> TDLSQRPRRLRKSPALRAMFEETTLSLNDLVLPIFVEEEIDDYKAVEAMPGVMRIPEKHLAREIERIANAGIRSVMTFGISHHTDETGSDAWREDGLVARMSRICKQTVPEMIVMSDTCFCEYTSHGHCGVLKEHGVDNDATLENLGKQAVVAAAAGADFIAPSAAMDGQVQAIRQALDAAGFKDTAIMSYSTKFASSFYGPFREAAGSALKGDRKSYQMNP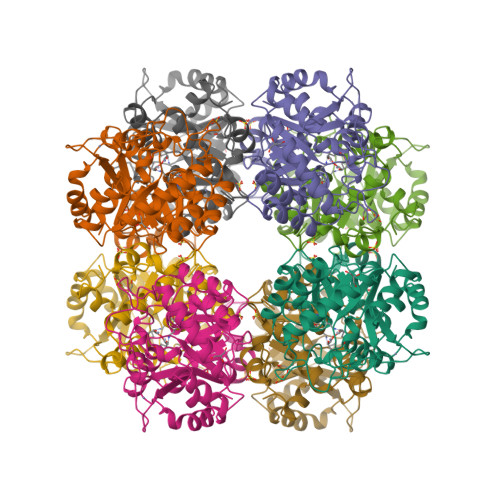MNRREAIRESLLDEAQGADCLMVKPAGAYLDIVRELRERTELPIGAYQVSGEYAMIKFAALAGAIDEEKVVLESLGSIKRAGADLIFSYFALDLAEKKILR> KRDPVY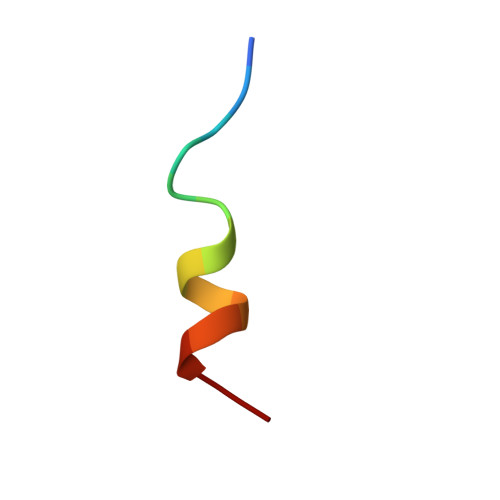FIKLSTIK>[2x]MASSPQRGRPRLNAARTTFVGDNGQPLRGPYTSTEWTAAAPYDQIARVKELGFNAVHLYAECFDPRYPAPGSKAPGYAVNEIDKIVERTRELGLYLVITIGNGANNGNHNAQWARDFWKFYAPRYAKETHVLYEIHNEPVAWGPPYSSSTANPPGAVDMEIDVYRIIRTYAPETPVLLFSYAVFGGKGGAAEALKDIRAFNKAVFGNENAVWTNEAVAFHGYAGWQETTIAVEELLKAGYPCFMTSYAGGAWGSGMGGLDVELTYELERLGVSWLTFQYIPPTGVSDDVTKPEYFSALVENSGLSWTPDYGNWPAARGVYGNGGLARETATWINNFLTGTTRIEAEDFDWGGNGVSYYDTDSVNVGGQYRPDEGVDIEKTSDTGGGYNVGWISEGEWLEYTIRVRNPGYYNLSLRVAGISGSRVQVSFGNQDKTGVWELPATGGFQTWTTATRQVFLGAGLQKLRINALSGGFNLNWIELSPILEHHHHHH

The GH5 arabinoxylanase (CtXyl5A) derived from Clostridium thermocellum displays an absolute requirement for xylans that contain Araf side chains. In this enzyme, the key specificity determinant is the Araf appended to O3 of the Xylp bound in the active site (−1 subsite). The dockerin domain recruits the enzyme into the cellulosome, a multienzyme plant cell wall degrading complex presented on the surface of C. thermocellum.

A third product complex was generated by co-crystallizing the nucleophile inactive mutant CtGH5E279S-CtCBM6 with a WAX-derived oligosaccharide. The data revealed a pentasaccharide bound to the enzyme, comprising β-1,4-xylotetraose with an Araf linked α-1,3 to the reducing end xylose. The xylotetraose was positioned in subsites −1 to −4 and the Araf in the −2* pocket. In the active site of CtXyl5A the α-d-Xylp, which is in its relaxed 4C1 conformation, makes the following interactions with the enzyme: O1 hydrogen bonds with the Nδ1 of His253 and Oϵ2 of Glu171 (catalytic acid-base) and makes a possible weak polar contact with the OH of Tyr255 and Oγ of Ser279 (mutation of the catalytic nucleophile); O2 hydrogen bonds with Nδ2 of Asn170 and OH of Tyr92. O3 (O1 of the Araf at the −2* subsite) makes a polar contact with Nδ2 of Asn139; the endocyclic oxygen hydrogens bonds with the OH of Tyr255. The Xylp in the active site makes strong parallel apolar interactions with Phe310. A surface representation of the enzyme shows that O3 and O2 of xylose units at subsites −2 to −4 are solvent-exposed and are thus available for decoration. Indeed, these pyranose sugars make very weak apolar interactions with the arabinoxylanase. At −2, Xylp makes planar apolar interactions with the Araf bound to the −2* subsite. Xylp at subsites −2 and −3, respectively, make weak hydrophobic contact with Val318, the −3 Xylp makes planar apolar interactions with Ala137, whereas the xylose at −4 forms parallel apolar contacts with Trp69.> MAAPAAEAPLSHVQQALAELAKPKDDPTRKHVCVQVAPAVRVAIAETLGLAPGATTPKQLAEGLRRLGFDEVFDTLFGADLTIMEEGSALLHRLTEHLEAHPHSDEPLPMFTSCCPGWIAMLEKSYPDLIPYVSSCKSPQMMLAAMVKSYLAEKKGIAPKDMVMVSIMPCTRKQSEADRDWFCVDADPTLRQLDHVITTVELGNIFKERGINLAELPEGEWDNPMGVGSGAGVLFGTTGGVMEAALRTAYELFTGTPLPRLSLSEVRGMDGIKETNITMVPAPGSKFEELLKHRAAARAEAAAHGTPGPLAWDGGAGFTSEDGRGGITLRVAVANGLGNAKKLITKMQAGEAKYDFVEIMACPAGCVGGGGQPRSTDKAITQKRQAALYNLDEKSTLRRSHENPSIRELYDTYLGEPLGHKAHELLHTHYVAGGVEEKDEKKSAWSHPQFEK

[FeFe]-hydrogenases represent one of natures’ most effective classes of redox enzymes catalyzing the reversible reduction of protons to dihydrogen (H2) at turnover frequencies of up to 9000 s-11–3. With their low catalytic over-potential, [FeFe]-hydrogenases represent excellent models for a regenerative and likewise economically feasible H2 production. Their active center (“H-cluster”) can be structured into a standard [4Fe-4S]-cluster ([4Fe]H) and a diiron site ([2Fe]H). Theoretical studies suggest that the most probable PT pathway comprises of strictly conserved residues E282, S319, E279, and C299 (from surface to H-cluster, numbering corresponds to CpI), including two protein-bound water molecules (Wat826, Wat1120 4XDC19, chain B) located between E279 and C29915,16,20. In this study, site-directed mutagenesis (SDM) is used to investigate the PT pathway of two [FeFe]-hydrogenases, namely CpI and HydA1, which represent the largest (M3) and smallest (M1) type of monomeric [FeFe]-hydrogenases, respectively.

Crystallization of HydA1 exclusively succeeded for apo-protein, which carries the [4Fe]H-cluster but lacks the [2Fe]H-site. Variants of HydA1 apo-protein were crystallized in space group P32 2 1, with a single chain in the asymmetric unit. However, comparisons of crystal structures of CpI apo- and holo-protein with apo-HydA1 demonstrated that a lack of cofactor does not affect the configuration of the putative PT pathway. In E282A, two water molecules occupy the space of the missing carboxylic acid group (chain B, Wat717 and Wat974). In the crystal structure of apo-E144AHydA1, one water molecule remains in a very similar position. It is therefore not surprising that both variants exhibit 50% wild-type activity. The pH-activity profile of E144AHydA1 was quite similar to wild-type HydA1, despite a flattening out of the local maximum at around pH 8. The latter suggests that this local activity maximum is depending on the presence of the surface-exposed Glu residue.>[2x]MGSSHHHHHHGSGLVPRGSAGMAAPGENRRVNADRLWDSLMEMAKIGPGVAGGNNRQTLTDADGEGRRLFQSWCEEAGLSMGVDKMGTMFLTRPGTDPDALPVHIGSHLDTQPTGGKFDGVLGVLSGLEAVRTMNDLGIKTKHPIVVTNWTNEEGARFAPAMLASGVFAGVHTLEYAYARKDPEGKSFGDELKRIGWLGDEEVGARK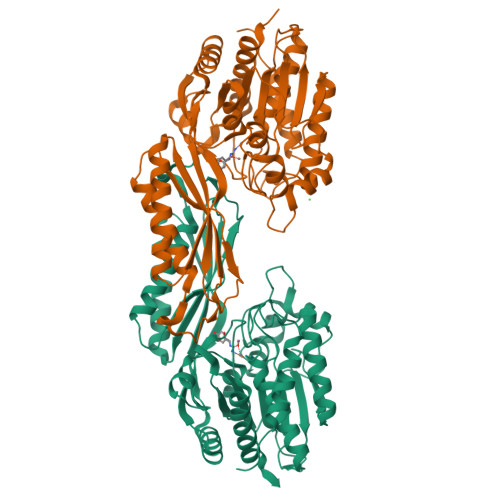MHAYFEYHIEQGPILEAENKQIGVVTHCQGGWWLEFTLTGREAHTGSTPMDMRVNAGLAMARILEMVQTVAMENQPGAVGGVGQMFFSPNSRNVLPGKVVFTVDIRSPDQAKLDGMRARIEAEAPKICERLGVGCSIEAVGHCDPVTFDPKLVETVRGAAEKLGYSHMNLVSGAGHDACWAAKVAPTTMIMCPCVGGLSHNEAEDISREWAAAGADVLFHAVLETAEIVE> E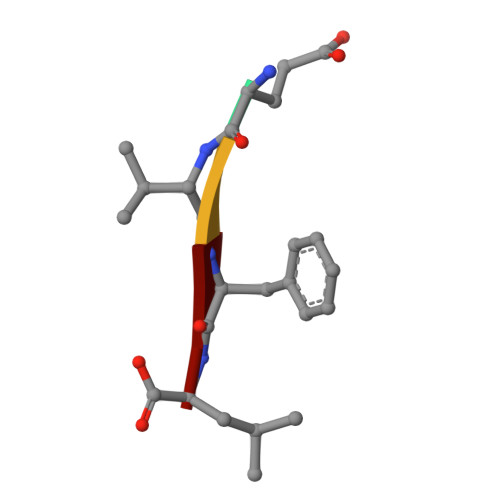VFL> SMSVKKPKRDDSKDLALCSMILTEMETHEDAWPFLLPVNLKLVPGYKKVIKKPMDFSTIREKLSSGQYPNLETFALDVRLVFDNCETFNEDDSDI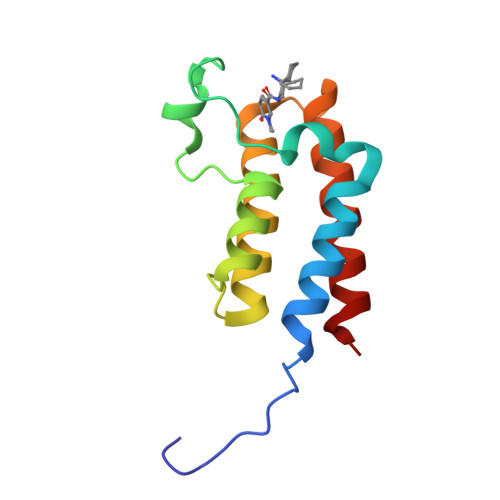GRAGHNMRKYFEKKWTDTFKVS> AAKALIVYGSTTGCTEYTAETIARELADAGYEVDSRDAASVEAGGLFEGFDLVLLGCSTWGDDSIELQDDFIPLFDSLEETGAQGR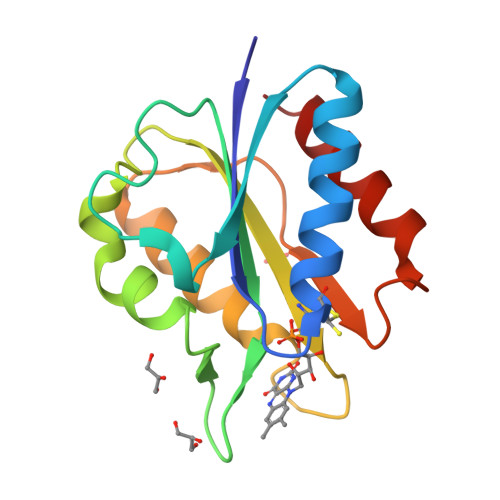KVACFGCGDSSWEYFCGAVDAIEEKLKNLGAEIVQDGLRIDGDPRAARDDIVGWAHDVRGAI> MSDLVTKFESLIISKYPVSFTKEQSAQAAQWESVLKSGQIQPHLDQLNLVLRDNTFIVSTLYPTSTDVH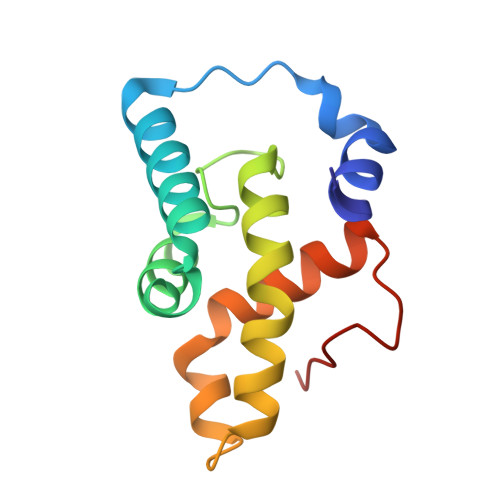VFEVALPLIKDLVASSKDVKSTYTTYRHILRWIDYMQNLLEVSSTDKLEINHD>[4x]GPLGSRIKTLSVSRPIIYGNTAKKMGSVKPPNAPAEHTHLWTIFVRGPQNEDISYFIKKVVFKLHDTYPNPVRSIEAPPFELTETGWGEFDINIKVYFVEEANEKVLN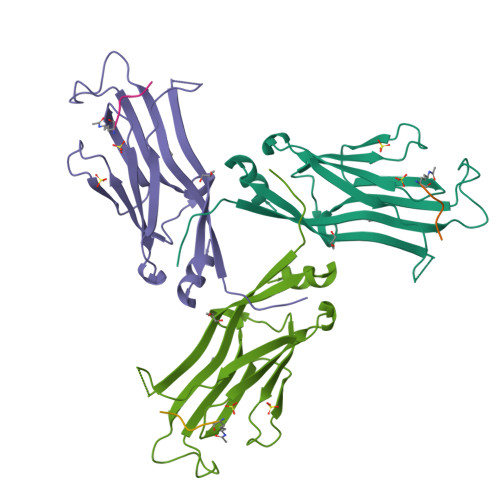FYHRLRLHPYANPVPNSDNGNEQNTTDHNSKDAEVSSVYFDEIVFNEPNEEFFKILMSRPG;>[4x]ATKAARKSAPA> GPLGSSKVSEQLKCCSGILKEMFAKKHAAYAWPFYKPVDVEALGLHDYCDIIKHPMDMSTIKSKLE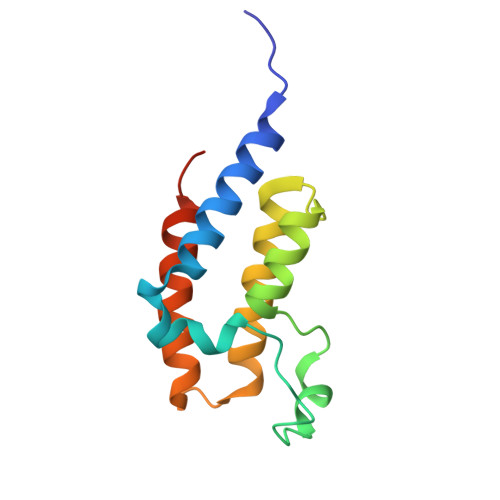AREYRDAQEFGADVRLMFSNCYKYNPPDHEVVAMARKLQDVFEMRFAKMPDEPEEP N-[(1E)-2-formyl-3-hydroxyprop-1-en-1-yl]-3-[(S)-sulfino]-D-valine | C9 H15 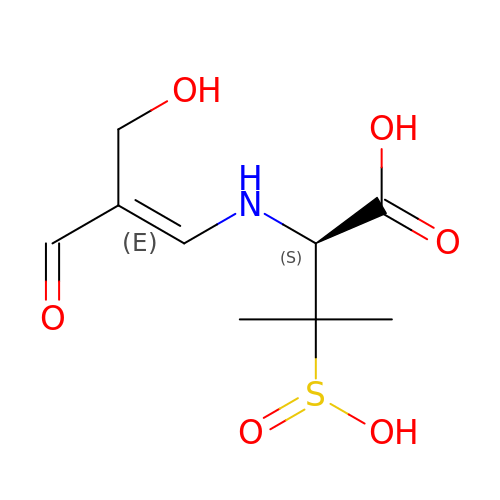N O6 S | RSKLLQJITLFPCX-NFNQMPKISA-N> NTYQFRNMIQCTVPSRSWWDFADYGCYCGCGSGTPVDDLDRCCQVHCNCYRQAGEISGCRPKFKTYTYECSGGTLTCKGDNNACAASSCDCDRLAAICFAGAPYNDNNYNIDLKARCN;> NIKQFNNMIQCTVPARSWWDFADYGCYCGSGSGSPVDDLDRCCQVHDNCYNAGGGVTGCAPKSKTYTYECSQGTLTCSGENSACAATVCDCDRLAAICF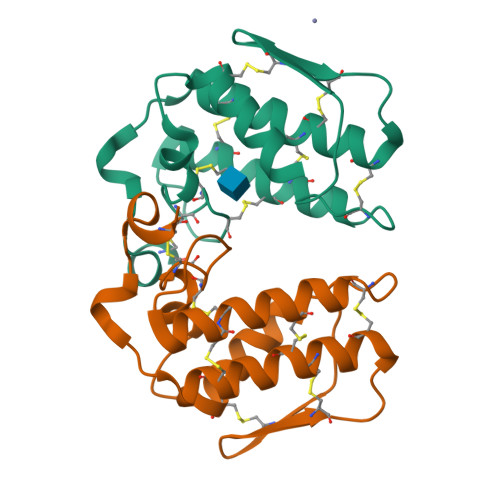AGAPYNDNNYNIDLKSRCQ>TEDEIRKLRKLLEEAEKKLYKLEDKTRRSEEISKTDDDPKAQSLQLIAESLMLIAESLLIIAISLLLSS[10x];>[2x]TEDEIRKLKKLLEEAEKKLYKLEDKTRRSEEISKTDDDPKAQSLQLIAESLMLI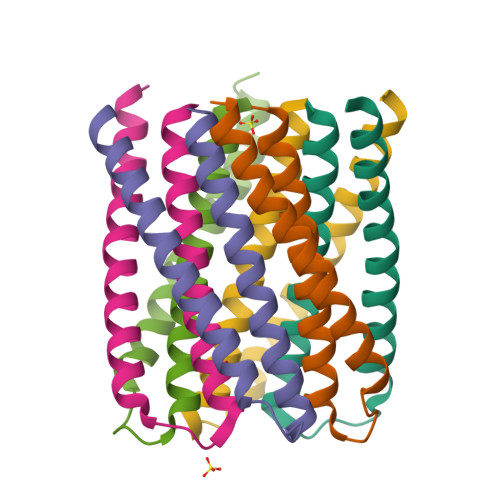AESLLIIAISLLLSS;>HHHHHHSGLVPRGSHM[2x]> EPALPSASEEQVAQDTEEVFRSYVFYRHQQEQEAEGVAAPADPEMVTLPLQPSSTMGQVGRQLAIIGDDINRRYDSEFQTMLQHLQPTAENAYEYFTKIATSLFESGINWGRVVALLGFGYRLALHVYQHGLTGFLGQVTRFVVDFMLHHC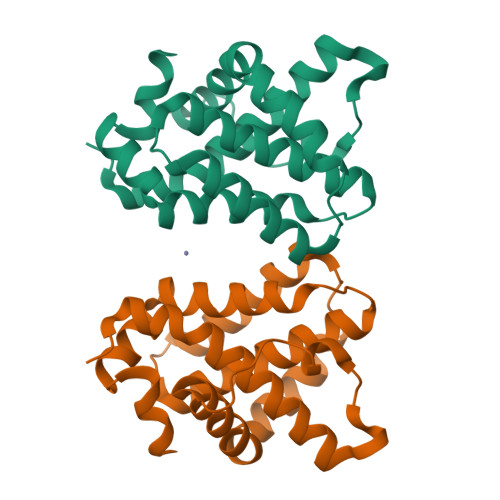IARWIAQRGGWVAALNLGNG> ALGSNSSSQPNRVARMPVDRNAPYYNMNHKHRGMAIIFNHEHFDIHSLKSRTGTNVDSDNLSKVLKTLGFKVTVFPNLKSEEINKFIQQTAEMDHSDADCLLVAVLTHGELGMLYAKDTHYKPDNLW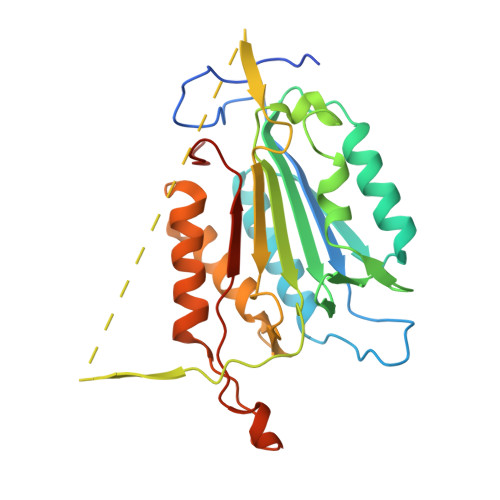YYFTADKCPTLAGKPKLFFIQACQGDRLDGGITLSRTETDGSPSTSYRIPVHADFLIAFSTVPGYFSWRNTTRGSWFMQALCEELRYAGTERDILTLLTFVCQKVALDFESNAPDSAMMHQQKQVPCITSMLTRLLVFGKKQSHL>[2x]MGSSHHHHHHSSGRENLYFQGHMVIIDNKHYLFIQKLGEGGFSYVDLVEGLHDGHFYALKRILCHEQQDREEAQREADMHRLFNHPNILRLVAYCLRERGAKH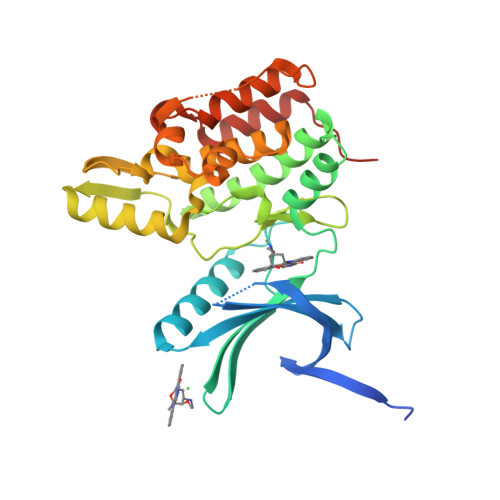EAWLLLPFFKRGTLWNEIERLKDKGNFLTEDQILWLLLGICRGLEAIHAKGYAHRDLKPTNILLGDEGQPVLMDLGSMNQACIHVEGSRQALTLQDWAAQRCTISYRAPELFSVQSHCVIDERTDVWSLGCVLYAMMFGEGPYDMVFQKGDSVALAVQNQLSIPQSPRHSSALWQLLNSMMTVDPHQRPHIPLLLSQLEALQPPAPGQHTTQIL> FFPSGTIAFFIFMMVFYAV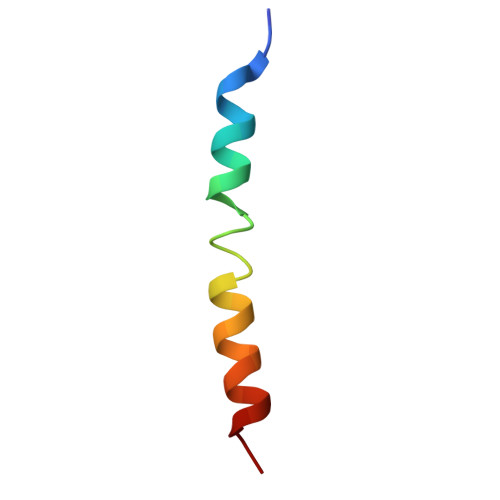LWFMIYWVLLERG The MRE11-RAD50-NBS1 (MRN) complex is a central, multifunctional factor in the detection, signaling and nucleolytic processing of DNA double-strand breaks (DSBs). The core MR complex contains two copies of both the ATPase RAD50 and the endo-/exonuclease MRE11, assembled in an elongated structure. This structure consists of a “head” module which includes MRE11 and the ATP binding cassette type nucleotide binding domains (NBDs) of RAD50, and a “tail” module formed by the coiled-coil domains (CCDs) of RAD50. Furthermore, MRN/X’s nuclease is highly regulated by trans-interacting factors that interact with a regulatory surface patch on RAD50, denoted “S site”.

The highest resolution structures were obtained by incubating MR or MH129NRN (nuclease dead mutant, hereafter referred to as ‘MRN’) with 50 bp DNA and ATP at 35 °C for 30 min, followed by addition of BeFx (producing the ATP mimic ADP•BeFx after ATP hydrolysis). Extensive processing resulted in 3D reconstructions with overall resolutions of 3.2 Å (MR) and 3.1 Å (MRN). The maps resolve MR’s and MRN’s catalytic head bound to DNA and parts of the CCD module, with ADP•BeFx•Mg2+ bound at both active sites. Human MR/MRN comprises two tightly engaged RAD50NBDs that bind into the concave side of the MRE11 dimer. The nuclease active site of MRE11 harbors density consistent with two Mn2+ ions (present in the buffer) but is shielded from any DNA access by the proximity of RAD50NBDs. DNA interacts with both RAD50NBDs in a two-fold symmetric manner, traversing the RAD50 dimer between the CCDs with a footprint of ~20 bases, consistent with ATP dependent DNA binding. The 3’ strand, as viewed from a DSB, binds to the RAD50NBD N-lobe along the top β-strand of the S site and to the subsequent α-helix, while the 5’ strand binds the N-lobe at a loop following the P-loop helix (Walker A motif). MRE11 does not substantially contribute to DNA binding in this state, with only a single residue (K467MRE11) at the HLH element in sufficient proximity to the 3’ strand. DNA interactions are virtually identical in MR and in MRN complexes. During 3D classification, we identified two separable conformational states in MR and MRN, one with the MRE11 dimer symmetrically attached to both RAD50NBDs, and one where the MRE11 catalytic domain dimer detaches as a rigid body from one RAD50NBD.

>[2x]MSRIEKMSILGVRSFGIEDKDKQIITFFSPLTILVGPNGAGKTTIIECLKYICTGDFPPGTKGNTFVHDPKVAQETDVRAQIRLQFRDVNGELIAVQRSMVCTQKSKKTEFKTLEGVITRTKHGEKVSLSSKCAEIDREMISSLGVSKAVLNNVIFCHQEDSNWPLSEGKALKQKFDEIFSATRYIKALETLRQVRQTQGQKVKEYQMELKYLKQYKEKACEIRDQITSKEAQLTSSKEIVKSYENELDPLKNRLKEIEHNLSKIMKLDNEIKALDSRKKQMEKDNSELEEKMEKVFQGTDEQLNDLYHNHQRTVREKERKLVDCHRELEKLNKESRLLNQEKSELLVEQGRLQLQADRHQEHIRARDSLIQSLATQLELDGFERGPFSERQIKNFHKLVRERQEGEAKTANQLMNDFAEKETLKQKQIDEIRDKKTGLGRIIELKSEILSKKQNELKNVKYELQQLEGSSDRILELDQELIKAERELSKAEKNSNVETLKMEVISLQNEKADLDRTLRKLDQEMEQLNHHTTTRTQMEMLTKDKADKDEQIRKIKSRHSDELTSLLGYFPNKKQLEDWLHSKSKEINQTRDRLAKLNKELASSEQNKNHINNELKRKEEQLSSYEDKLFDVCGSQDFESDLDRLKEEIEKSSKQRAMLAGATAVYSQFITQLTDENQSCCPVCQRVFQTEAELQEVISDLQSKLRLAPDKLKSTESELKKKEKRRDEMLGLVPMRQSIIDLKEKEIPELRNKLQNVNRDIQRLKNDIEEQETLLGTIMPEEESAKVCLTDVTIMERFQMELKDVERKIAQQAAKLQGIDLDRTVQQVNQEKQEKQHKLDTVSSKIELNRKLIQDQQEQIQHLKSTTNELKSEKLQISTNLQRRQQLEEQTVELSTEVQSLYREIKDAKEQVSPLETTLEKFQQEKEELINKKNTSNKIAQDKLNDIKEKVKNIHGYMKDIENYIQDGKDDYKKQKETELNKVIAQLSECEKHKEKINEDMRLMRQDIDTQKIQERWLQDNLTLRKRNEELKEVEEERKQHLKEMGQMQVLQMKSEHQKLEENIDNIKRNHNLALGRQKGYEEEIIHFKKELREPQFRDAEEKYREMMIVMRTTELVNKDLDIYYKTLDQAIMKFHSMKMEEINKIIRDLWRSTYRGQDIEYIEIRSDADENVSASDKRRNYNYRVVMLKGDTALDMRGRCSAGQKVLASLIIRLALAETFCLNCGIIALDEPTTNLDRENIESLAHALVEIIKSRSQQRNFQLLVITHDEDFVELLGRSEYVEKFYRIKKNIDQCSEIVKCSVSSLGFNVH;>MSTADALDDENTFKILVATDIHLGFMEKDAVRGNDTFVTLDEILRLAQENEVDFILLGGDLFHENKPSRKTLHTCLELLRKYCMGDRPVQFEILSDQSVNFGFSKFPWVNYQDGNLNISIPVFSIHGNHDDPTGADALCALDILSCAGFVNHFGRSMSVEKIDISPVLLQKGSTKIALYGLGSIPDERLYRMFVNKKVTMLRPKEDENSWFNLFVIHQNRSKHGSTNFIPEQFLDDFIDLVIWGHEHECKIAPTKNEQQLFYISQPGSSVVTSLSPGEAVKKHVGLLRIKGRKMNMHKIPLHTVRQFFMEDIVLANHPDIFNPDNPKVTQAIQSFCLEKIEEMLENAERERLGNSHQPEKPLVRLRVDYSGGFEPFSVLRFSQKFVDRVANPKDIIHFFRHREQKEKTGEEINFGKLITKPSEGTTLRVEDLVKQYFQTAEKNVQLSLLTERGMGEAVQEFVDKEEKDAIEELVKYQLEKTQRFLKERHIDALEDKIDEEVRRFRETRQKNTNEEDDEVREAMTRARALRSQSEESASAFSADDLMSIDLAEQMANDSDDSISAATNKGRGRGRGRRGGRGQNSASRGGSQRGRADTGLETSTRSRNSKTAVSASRNMSIIDAFKSTRQQPSRNVTTKNYSEVIEVDESDVEEDIFPTTSKTDQRWSSTSSSKIMSQSQVSKGVDFESSEDDDDDPFMNTSSLRRNRRSGGSLEVLFQGPDYKDDDDKGTDYKDDDDK[2x]> SPQLEELITKVSKAHQETFPSLCQLGKYTTNSSADHRVQLDLGLWDKFSELATKCIIKIVEFAKRLPGFTGLSIADQITLLKAACLDILMLRICTRYTPEQDTMTFSDGLTLNRTQMHNAGFGPLTDLVFAFAGQLLPLEMDDTETGLLSAICL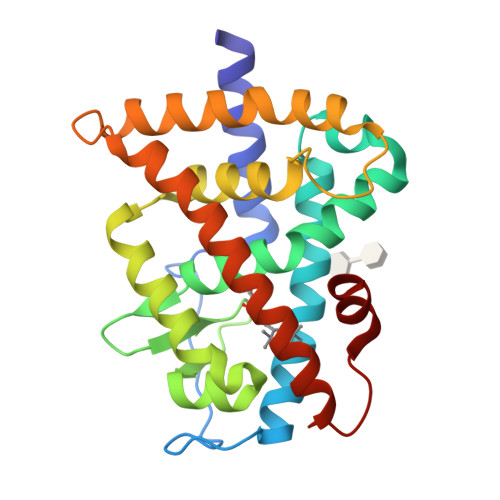ICGDRMDLEEPEKVDKLQEPLLEALRLYARRRRPSQPYMFPRMLMKITDLRGISTKGAERAITLKMEIPGPMPPLIREMLE>GAPPAPALRIDYP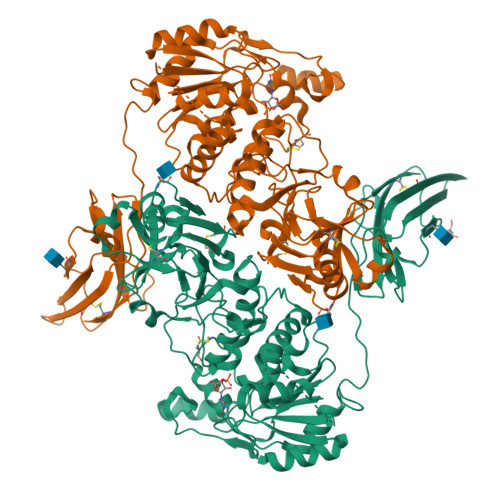KALQILTEGGTHMVCTGRTHTDRLCRFKWLCYSSEAEEFIFFHGNASVMLPSLGSRRFQPALLDLSTVEDHNTQYFNFVELPAAALRFMPKPVFVPDVALIANRFNPDNLMHVFHDDLLPLFYTLRQFPGLAREARLFFMEGWGEGAHFDLYKLLSPKQPLLRAQLKALGRLLCFSHAFVGLSKVTTWYQYGFVQPQGPKANILVSGNEIRQFAHFLMEKLNVSQAGGPLGEEYILVFSRTQNRLILNEAELLLALAQEFQMKTVTVSLEDHAFADVVRLVSNASMLVSMHGAQLVTALFLPRGAAVVELFPYAVNPDHYTPYKTLATLPGMDLQYIAWQNTMPENTVTHPERPWDQGGIAHLDRAEQARILQSREVPRHLCCRNPEWLFRIYQDTKVDIPSLIQTIRRVVKGHPGPRKQKWTVSLYPGKVREARCQASVQGASEARLSVSWQIPWNLKYLKVREVKYEVWLQEQGENTYVPYMLALQNHTFTENIKPFTTYLVWIRCIFNKTLLGPFADVLVCST[2x]> MASKSKVDNQFYSVEVGDSTFTVLKRYQNLKPIGSGAQGIVCAAYDAVLDRNVAIKKLSRPFQNQTHAKRAYRELVLMKCVNHKNIISLLNVFTPQKTLEEFQDVYLVMELMDANLCQVIQMELDHERMSYLLYQMLCGIKHLHSAGIIHRDLKPSNIVVKSDCTLKILDFGLARTAGTSFMMTPYVVTRYYRAPEVILGMGYKENVDIWSVGCIMGEMVRHKILFPGRDYIDQWNKVIEQLGTPCPE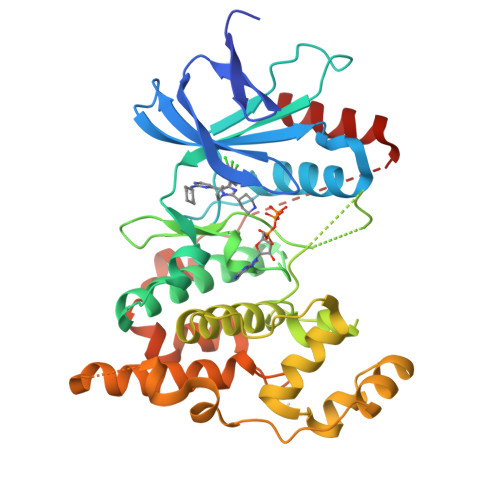FMKKLQPTVRNYVENRPKYAGLTFPKLFPDSLFPADSEHNKLKASQARDLLSKMLVIDPAKRISVDDALQHPYINVWYDPAEVEAPPPQIYDKQLDEREHTIEEWKELIYKEVMNS>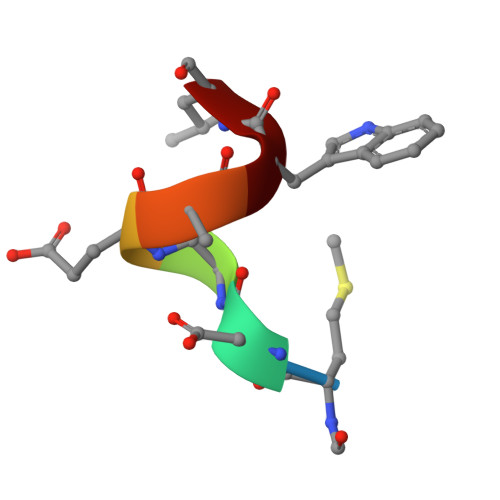 MDVEAWL>[2x]QYLLPEAKAQDSDKICVVINLDETLVHSSFKPVNNADFIIPVEIDGVVHQVYVLKRPHVDEFLQRMGELFECVLFTASLAKYADPVADLLDKWGAFRARL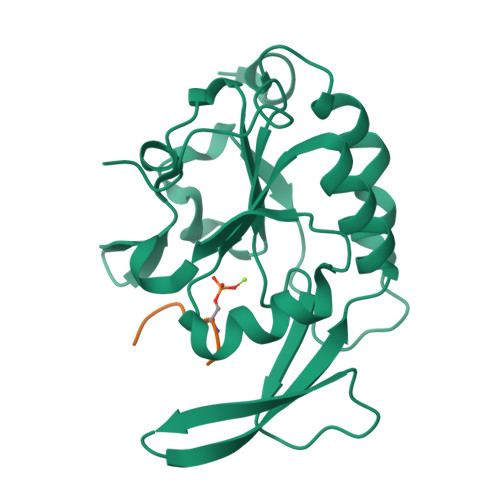FRESCVFHRGNYVKDLSRLGRDLRRVLILDNSPASYVFHPDNAVPVASWFDNMSDTELHDLLPFFEQLSRVDDVYSVLRQ;>EDLSPPSPPLPK[2x]>[2x]MIIHIVGGGPRELLPDLRFYDGEDVCWVGVDRGTMTLLEAGFRP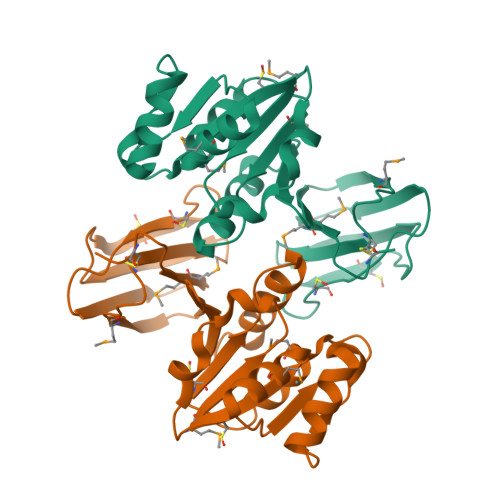VRAFGDFDSLPAEDVVKLQQAFPDLDVWPAEKDKTDMEIALDWAVEQTARCIRLFGATGGRLDHLFGNVELLLKYADRPIEIVDRQNVLTVHLPGTYTVMYDARYCYVSYIPVSETVAEFTLTGFKYPLTNCHISRGSTLCISNELIQSSGTFSFSEGILMMIRSSDSSCLLEHHHHHH6-azanyl-11-methyl-2-oxidanylidene-N-(pyridin-3-ylmethyl)-1,7,9-triazatricyclo[8.4.0.0^3,8]tetradeca-3(8),4,6,9,11,13-hexaene-5-carboxamide 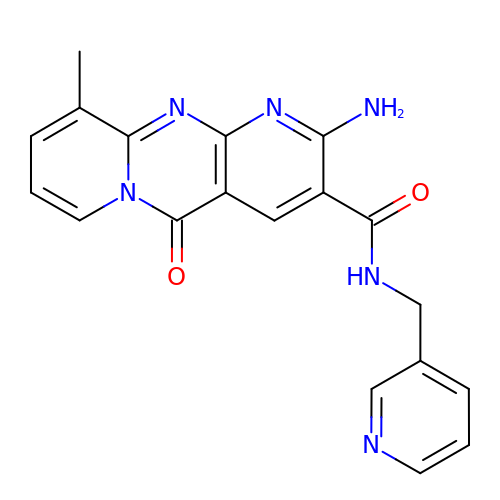| C19 H16 N6 O2 | FDRSMDXOIMNVLE-UHFFFAOYSA-N>MSASDGQGMRAVILVGGFGTRLRPLTLTTPKPLVPFCNKPMIIHQIEALKAVGVTEVILAVAYRPEAMKEQMDEWSRKLGVSFVFSVEEEPLGTAGPLALARDILMQDDKPFFVLNSDVTCTFPMQELLDFHKAHGGEGTIMVSQVTQWEKYGVVVYSPQNYQIERFVEKP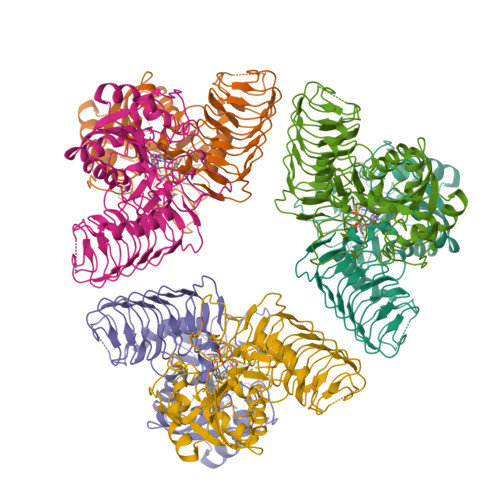SRFLGDRINAGIYIFNKSILDRIPPRRASIEKEIFPAMAAEGQLYAFNLEGFWMDVGQPKDYILGMTKFIPSLVHGNRETEQLHTEAVEHQRGGRFTVIGASLIDPSAKIGDGAVIGPYASIGANCVIGESCRIDNAAILENSKVGKGTMVSRSIVGWNNRIGSWCHIKDISVLGDDVEVKDGVILIGTKVLPNKDVGEHRFEPGIIM[6x]> GSHMGLFNAHAVAQQRADRIATLLQSFADGQLDTAVGEAPAPGYERHYDSLRALQRQLREQRAELQQVESLEAGLAEMSRQHEAGWIDQTIPAERLEGRAARIAKGVNELVAAHIAVKMKVVSVVTAYGQGNFEPLMDRLPGKKAQITEAIDGVRERLRGAAEATSAQLATAAYN

HAMP domains are small modules, approximately 50 amino acids, that dimerize to form an entirely parallel four-helix bundle with two helices (AS1 and AS2) supplied from each subunit. A semi-structured connector separates the AS1 and AS2 helices and contains two conserved hydrophobic residues, termed HR1 and HR2. Aer2 is a soluble receptor that contains three N-terminal HAMP domains, a gas-sensing, heme-containing PAS domain, two additional HAMP domains, and an MCP KCM. The three N-terminal HAMP domains of Aer2 (named HAMP1, HAMP2, and HAMP3 from N- to C-terminus) provide examples of two distinctly different conformations: HAMP1 and HAMP3 are similar to the Af1503 NMR structure, whereas HAMP2 has a comparatively distorted four-helix bundle structure in which the AS2 helices approximate a two-helix coiled coil and the AS1 helices splay outward at the C-terminal end.

Notable was the L44H mutation, which generated a CW lock (i.e., exclusively tumbling) phenotype in both CheRB+ and CheRB− cells. Crystals of L44H and V33G proteins were obtained in the context of Aer2 1–172 using conditions similar to those of the native protein. The L44H mutation modified the HAMP1 domain structure while leaving the poly-HAMP2/3 domains largely unchanged. The His44 side chain redirected from the bundle core towards AS1. This caused a tilt in the AS1 helix and a 5 Å shift at the top of AS1, resulting in a loss of secondary structure at the AS1 N-terminus. Despite these adjustments in AS1, the AS2 output helices superimposed with those of the native HAMP1 structure. In other words, the mutation did not alter the position of the HAMP1 AS2 helices, which must transmit the CW downstream signal. In the L44H structure, the tilt of AS1 drives the helices apart, disrupting upstream helical packing and resulting in a loss of observed secondary structure at the N-terminus of AS1. In the context of a transmembrane MCP, if this helix disruption were maintained, it would decouple TM2 from AS1. Because the L44H variant is strongly CW biasing, and the H1 conformation generates CW output, we assume that the structure seen at the C-terminal domain in the crystal is maintained in the Tar fusions.> EXCQKWMWTCDSARACCEGLRC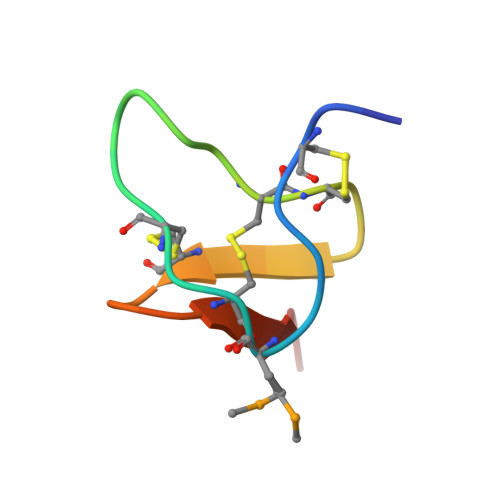KLWCRKEIX> GSPEFIEKNFVITDPRLPDNPIIFASDGFLELTEYSREEILGR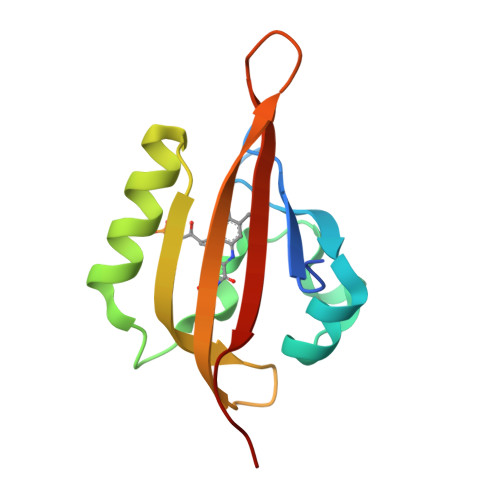NARFLQGPETDQATVQKIRDAIRDQRETTVQLINYTKSGKKFWNLLHLQPVRDQKGELQYFIGVQLDGSDHV> MNVGDRVRVTSSVVVYHHPEHAK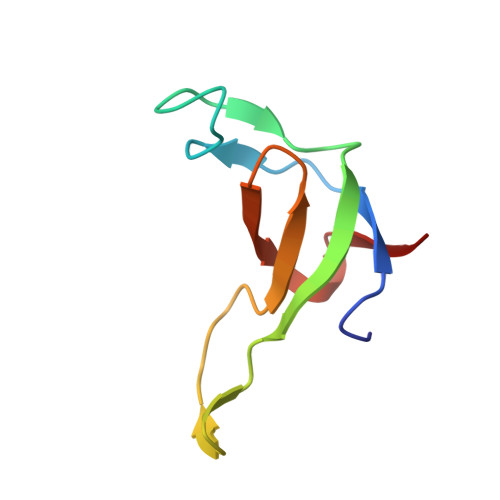TAFDLQGMEGEVAAVLTGWQGRPISANLPVLVKFEQRFKAHFRPDEVTLI> MNLPTAQEVQGLMARFIELVDVGDIEA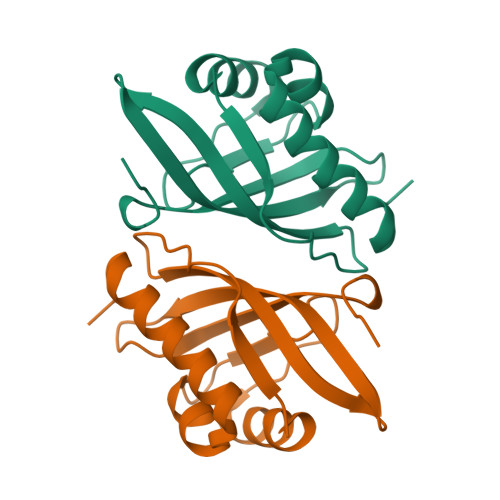IVQMYADDATVEDPFGQPPIHGREQIAAFYRQGLGGGKVRACLTGPVRASHNGCGAMPFRVEMVWNGQPCALDVIDVMRFDEHGRIQTMQAYWSEVNLSVREPQ> MKEKIRKKILLAPEEPGVYIFKNKGVPIYIGKAKRL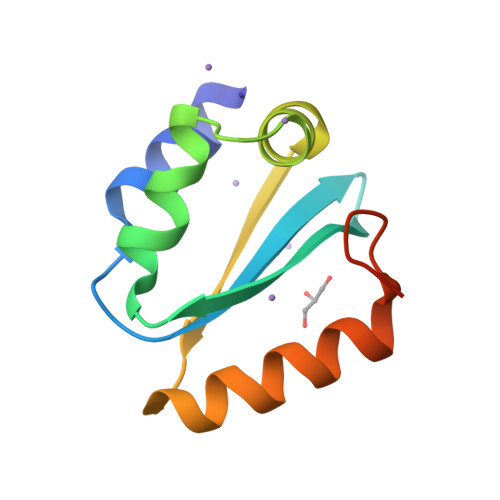SNRLRSFLNPQTEKVFRIGEEADELETIVVMNEREAFILEANLIKKYRPKYNVRLKDTDF> MIASKKGKEMLLTLSPIYEQSIIMQ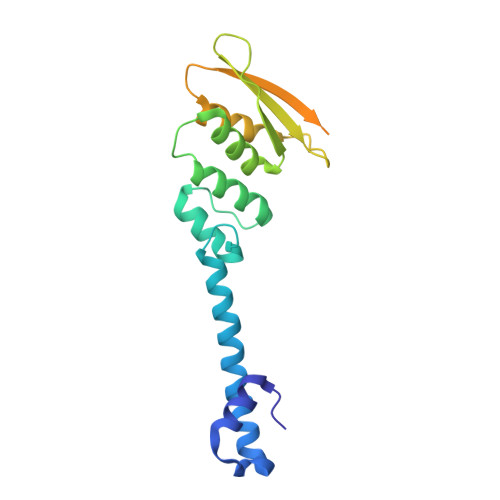SLYEAIGSEFDNLELLDEEIELQLFPQSATWGLGFWENRVGLITNLDEDMETRRRKVIAKLQSKYIMTPKRMSMILQSYTGANIKINENISPYTFGVELTSTQGFPKDLEDLYKRVNVIKPSHLAVSYKLVSLLKSKTYFAQTAIMSEEITIYPYTSKEVKASVKAKFALAHNMSSETLTVYPR> MPFEVVFDGAKEFADLIATASNLIDEAAFKFTEEGISMRAMDPSRVVLIDLNLPESIFSKYEVEEPETIGINMDQFKKILKRGKAKDTLILRKGDENFLEITFEGTAKRTFRLPLIDVEELELELPELPFTAKVVLLGEVLKEGIKDASLVSDAIKFIAKENEFTMKAEGETNEVEIRLTLEDEGLLDLEVEEETKSAYGIRYLSDMVKGIGKADEVILRFGNEMPLQMEYMIRDEGRLTFL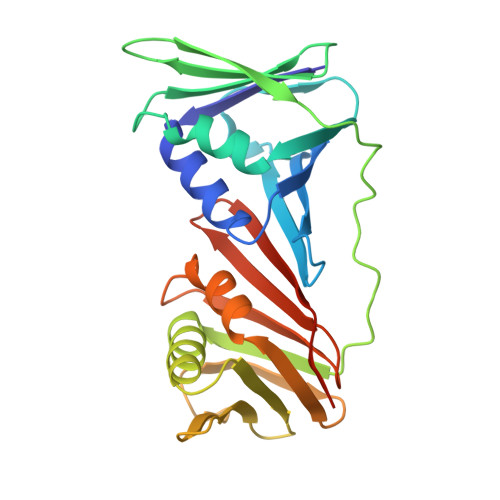LAPRVEEHHHHHH>[2x]MMFKRAIIFTSFNGFEKVSRTEKRRLAKIINARVSIIDEYLRA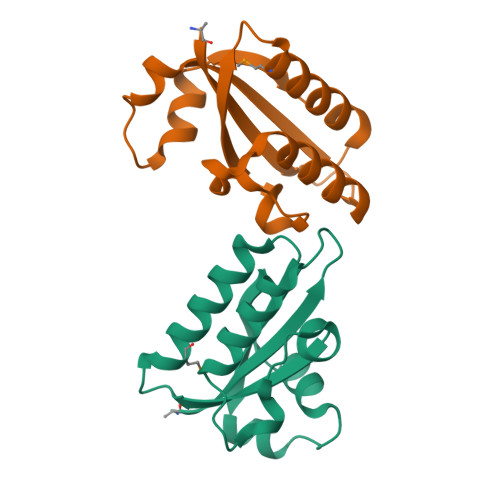KDTNASLDGQYRAFLFNDESPAMTEFLAKLKAFAESCTGISIDAWEIEESEYVRLPVERRDFLAAANGKEIFKI> MTEETISQAVPPVRDWPAVDLPGSDFDPVLTELMREGPVTRISLPNGEGWAWLVTRHDDVRLVTNDPRFGREAVMDRQVTRLAPHFIPARGAVGFLDPPDHTRLRRSVAAAFTARGVERVRERSRGMLDELVDAMLRAGPPADLTEAVLSPFPIAVICELMGVPATDRHSMHTWTQLILSSSHGAEVSERAKNEMNAYFSDLIGLRSDSAGEDVTSLLGAAVGRDEITLSEAVGLAVLLQIGGEAVTNNSGQMFHLLLSRPELAERLRSEPEIRPRAIDELLRWIPHRNAVGLSRIALEDVEIKGVRIRAGDAVYVSYLAANRDPEVFPDPDRIDFERSPNPHVSFGFGP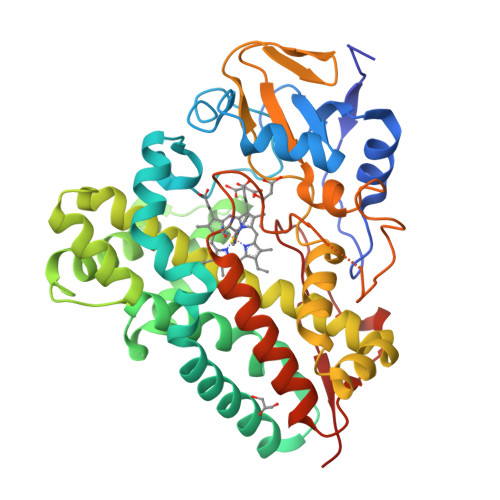HYCPGGMLARLESELLVDAVLDRVPGLKLAVAPEDVPFKKGALIRGPEALPVTWHA>[4x]SN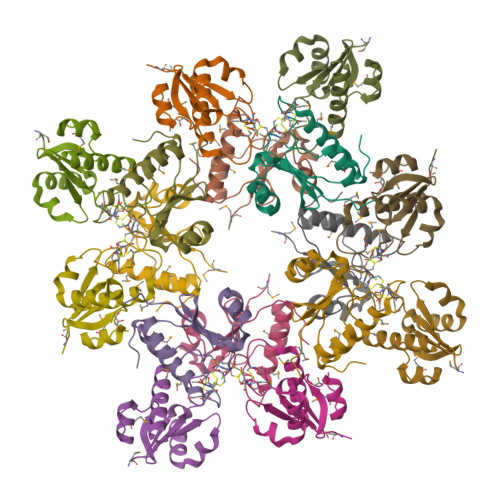AMKKIEIFDPAMCCPTGLCGTNINPELMRIAVVIESLKKQGIIVTRHNLRDEPQVYVSNKTVNDFLQKHGADALPITLVDGEIAVSQTYPTTKQMSEWTGVNLD> VVGGTEAQRNSWPSQISLQYRSGSSWAHTCGGTLIRQNWVMTAAHCVDRELTFRVVVGEHNLNQNNGTEQYVGVQKIVVHPYWNTDDVAAGYDIALLRLAQSVTLNSYVQLGVLPRAGTILANNSPCYITGWGLTRTNGQLAQTLQQAYLPTVDYAICSSSSYWGSTVKNSMVCAGGDGVRSGCQGDSGGPLHCLVNG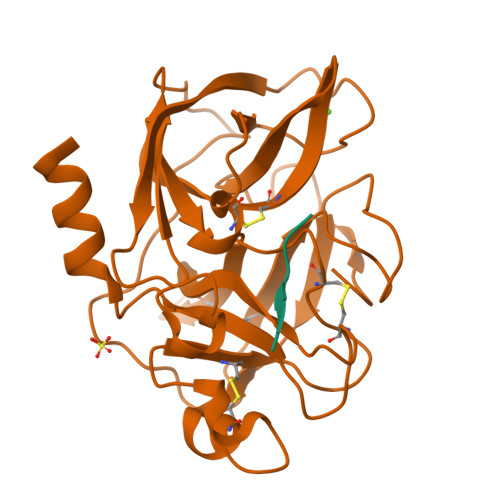QYAVHGVTSFVSRLGCNVTRKPTVFTRVSAYISWINNVIASN;> YPFVEPIKA> HHHHHHGSANKAVNDFILAMNYDKKKLLTHQGESIENRFIKEGNQLPDEFVVIERKKRSLSTSTSDISVTATNDSRLYPGALLVVDETLLENNPTLLAVDRAPMTYSIDLPGLASSDSFLQVEDPSNSSVRGAVNDLLAKWHQDYGQVNNVPARMQYEKITAHSMEQLKVKFGSDFEKTGNSLDIDFNSVHSGEKQIQIVNFKQIYYTVSVDAVRNPGDVFQDTVTVEDLKQRGISAERPLVYISSVAYGRQVYLKLETTSKSDEVEAAFEALIKGVKVAPQTEWKQILDNTEVKAVILGGDPSSGARVVTGKVDMVDDLIQEGSRFTADHPGLPISYTTSFLRDNVVATFQNSTDYVETKVTAYRNGDLLLDHSGAYVAQYYITWDELSYDHQGKEVLTPKAWDRNGQDLTAHFTTSIPLKGNVRNLSVKIRECTGLAWEWWRTVYEKTDLPLVRKRTISIWGTTLYPQVEDKVEN

Pneumolysin (PLY), a major virulence factor of the bacterium, is a pore-forming toxin belonging to the family of cholesterol-dependent cytolysins (CDCs). PLY is produced as a water-soluble monomer and recognises mammalian cells via its C-terminal domain (domain 4) before assembling into circular prepores of ~30–50 monomers on the surface of cholesterol-rich membranes. The monomers in the prepore undergo critical structural changes, including the unfurling of two alpha helical bundles (α-HB1 and α-HB2) in domain 3 in each monomer that are then refolded into β-hairpins (transmembrane hairpins TMH1 and TMH2) for insertion into the membrane, which is facilitated by a structural collapse towards the membrane surface. The resultant PLY β-barrel pore has a diameter of ~300 Å that causes lysis of the target cell.

PLY adopts the canonical CDC fold with maximal dimensions of 123 Å by 20 Å by 49 Å. The most significant difference between PLY and the other CDCs is that it adopts a linear shape down its long axis whereas the other CDCs tend to be bent to various degrees due to different orientations of D4 with respect to the rest of the molecule. A significant difference, not observed in any of the published CDC structures, is the high mobility of regions of two strands (residues 29 to 35, 46 to 50) in D2. Consequently, the hydrogen bond interactions that D2 forms with both D3 and D4 that are typically observed in SLY and other CDCs are absent in PLY. Two gold cyanide compounds, used to improve the quality of the crystals, are bound to Cys 428. In one site the gold complex packs against Trp 435 and Trp 436 and the other packs against Tyr 461 from a symmetry related molecule. The Trp-rich loop in PLY D4 (residues 427 to 437) adopts the same conformation as that previously seen in SLY and SLO, despite the binding of the gold complex to Cys 428. The monomers in the crystal are tightly packed in an elongated linear arrangement. The buried surface between PLY subunits is extensive, with more than 1500 Å2 buried in the interface (750 Å2 from one monomer and 770 Å2 from the second). Thus it seems the linear oligomers observed in the ILY, LLO and PLY structures are glimpses of the very early stages of weaker monomer-monomer interactions required before the interactions become strong enough to drive the conformational changes needed to induce circularisation of the oligomer.>EYGDLHLFGPNQRPAPCYDPCEAVLVESIPEGLDFPNASTGNPSTSQAWLGLLAGAHSSLDIASFYWTLTNNDTHTQEPSAQQGEEVLRQLQTLAPKGVNVRIAVSKPSGPQPQADLQALLQSGAQVRMVDMQKLTHGVLHTKFWVVDQTHFYLGSANMDWRSLTQVKELGVVMYNCSCLARDLTKIFEAYWFLGQAGSSIPSTWPRFYDTRYNQETPMEICLNGTPALAYLASAPPPLCPSGRTPDLKALLNVVDNARSFIYVAVMNYLPTLEFSHPHRFWPAIDDGLRRATYERGVKVRLLISCWGHSEPSMRAFLLSLAALRDNHTHSDIQVKLFVVPADEAQARIPYARVNHNKYMVTERATYIGTSNWSGNYFTETAGTSLLVTQNGRGGLRSQLEAIFLRDWDSPYSHDLDTSADSVGNACRLLAAQ[2x]

PLD3 is synthesized as a type II transmembrane protein and proteolytically cleaved in lysosomes, yielding a soluble active form. The deficiency of PLD3 leads to the slowed degradation of nucleic acids in lysosomes and chronic activation of nucleic acid-specific intracellular toll-like receptors. PLD3 has a typical phospholipase fold and forms homodimers with two independent catalytic centers via a newly identified dimerization interface. While crystal structures for RNaseT2 and DNase II are available and provide important insight into the molecular details and function of both enzymes, no experimentally determined structural information is available for the 5′ exonucleases PLD3 or PLD4. Both PLD3 and PLD4 belong to the phospholipase-D (PLD) family of phosphodiesterases, a protein family that shares a common biochemical mechanism and an H(X)K(X4)D (HKD) signature motif within their active site.

To obtain structural information, crystals of hPLD3 in the presence of the identified ss T*TCATG oligomer were grown and diffracted to 1.8 Å. The hPLD3 structure co-crystallized with the ssDNA phosphorothioate (*) modified T*TCATG oligomer revealed a partly visible DNA sequence bound within the central active site. The 5′ end of the first thymidine and the phosphorothioate group of the second thymidine were bound in the active site. The phosphorothioate was coordinated by six hydrogen bonds within the HKD/HKE motif involving the active site residues His201, Lys203, Asn218, His416, Lys418, and Asn432. The thymidine was hydrophobically stacked against Tyr411 and was further stabilized by a hydrogen bond with Tyr126 (protomer A) or water-mediated contacts via Asp220 (protomer B) to the thymidine O2. The O5 of the deoxyribose was bound by the Tyr411 together with an alternative conformation of His416 (in protomer B) and water-mediated by Asp220 (protomer A). The remaining nucleotides of the T*TCATG oligo were not visible in the electron density. Crystals for hPLD3 in complex with T*TCATG were grown in a crystallization condition containing sodium iodite. It has recently been reported that iodine preferentially attacks sulfur in phosphorothioate DNA and induces nucleolytic cleavage. Therefore, the bound 3′-phosphorothioate thymidine in the active site is most likely the cleavage product of T*TCATG, which further underlines the 5′-exonuclease function of hPLD3.>GPLSLSVDAFKILEDPKWEFPRKNLVLGKTLGEGEFGKVVKATAFHLKGRAGYTTVAVKMLKENASPSELRDLLSEFNVLKQVNHPHVIKLYGACSQDGPLLLIVEYAKYGSLRGFLRESRKVGPGYLGSGGSRNSSSLDHPDERALTMGDLISFAWQISQGMQYLAEMKLVHRDLAARNILV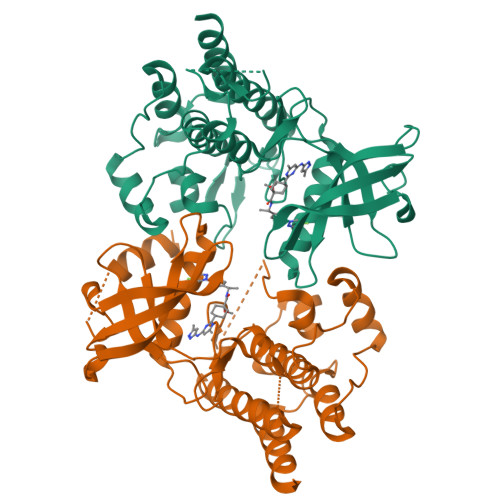AEGRKMKISDFGLSRDVYEEDSYVKRSQGRIPVKWMAIESLFDHIYTTQSDVWSFGVLLWEIVTLGGNPYPGIPPERLFNLLKTGHRMERPDNCSEEMYRLMLQCWKQEPDKRPVFADISKDLEKMMVKRR[2x]> MASNLVEMFNAAL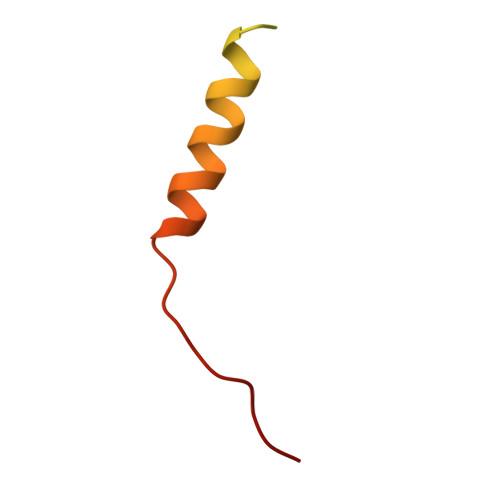NWVTMILESPSARVVLFGVPIRGHFFVEGLLGVVIIILLTRKSYKPPKR>[4x]SRPLSDQEKRKQISVRGLAGVENVTELKKNFNRHLHFTLVKDRNVATPRDYYFALAHTVRDHLVGRWIRTQQHYYEKDPKRIYYLSLEFYMGRTLQNTMVNLALENACDEATYQLGLDMEELEEIEEDAGLGNGGLGRLAACFLDSMATLGLAAYGYGIRYEFGIFNQKICGGWQMEEADDWLRYGNPWEKARPEFTLPVHFYGRVEHTSQGAKWVDTQVVLAMPYDTPVPGYRNNVVNTMRLWSAKAPNDF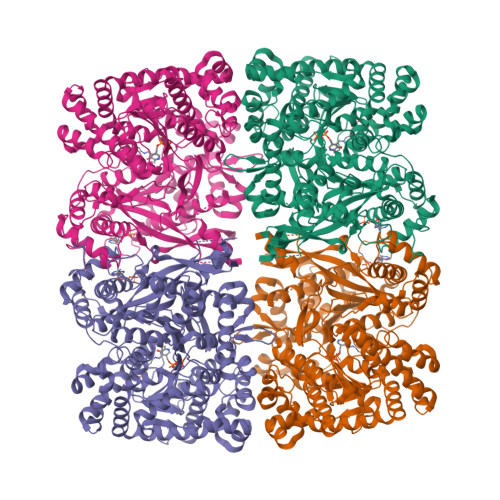NLKDFNVGGYIQAVLDRNLAENISRVLYPNDNFFEGKELRLKQEYFVVAATLQDIIRRFKSSKFGCRDPVRTNFDAFPDKVAIQLNDTHPSLAIPELMRVLVDLERLDWDKAWEVTVKTCAYTNHTVLPEALERWPVHLLETLLPRHLQIIYEINQRFLNRVAAAFPGDVDRLRRMSLVEEGAVKRINMAHLCIAGSHAVNGVARIHSEILKKTIFKDFYELEPHKFQNKTNGITPRRWLVLCNPGLAEIIAERIGEEYISDLDQLRKLLSYVDDEAFIRDVAKVKQENKLKFAAYLEREYKVHINPNSLFDVQVKRIHEYKRQLLNCLHVITLYNRIKKEPNKFVVPRTVMIGGKAAPGYHMAKMIIKLITAIGDVVNHDPVVGDRLRVIFLENYRVSLAEKVIPAADLSEQISTAGTEASGTGNMKFMLNGALTIGTMDGANVEMAEEAGEENFFIFGMRVEDVDRLDQRGYNAQEYYDRIPELRQIIEQLSSGFFSPKQPDLFKDIVNMLMHHDRFKVFADYEEYVKCQERVSALYKNPREWTRMVIRNIATSGKFSSDRTIAQYAREIWGVEPSRQRLPAPDEKIP>MGSSHHHHHHENLYFQSMASMKTELIRTISLYDTI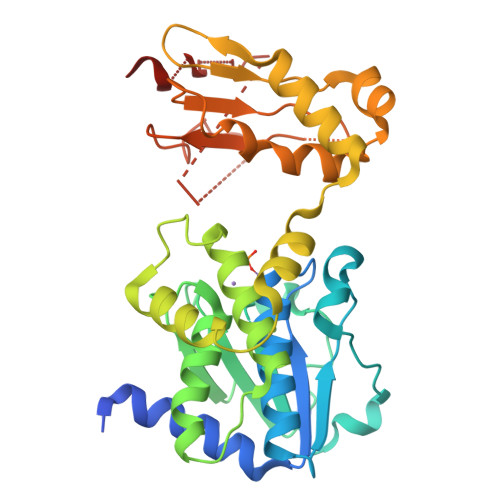ILHRHVRPDPDAYGSQCGLTEILRETYPEKNIFAVGTPEPSLSFLYSLDEVDNETYEGALVIVCDTANQERIDDQRYPSGAKLMKIDAHPNEDPYGDLLWVDTSASSVSEMIYELYLEGKEHGWKLNTKAAELIYAGIVGDTGRFLFPNTTEKTLKYAGELIQYPFSSSELFNQLYETKLNVVKLNGFIFQNVSLSENGAASVFIKKDTLEKFGTTASEASQLVGTLGNISGIRAWVFFVEEDDQIRVRFRSKGPVINGLARKYNGGGHPLASGASIYSWDEADRILADLETLCKEHE[4x]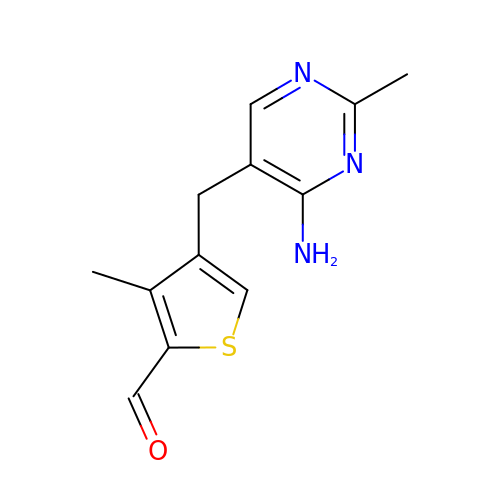4-[(4-amino-2-methylpyrimidin-5-yl)methyl]-3-methylthiophene-2-carbaldehyde | C12 H13 N3 O S | NWGVSSQLYKZANM-UHFFFAOYSA-N>[2x]MAEVIRSSAFWRSFPIFEEFDSETLCELSGIASYRKWSAGTVIFQRGDQGDYMI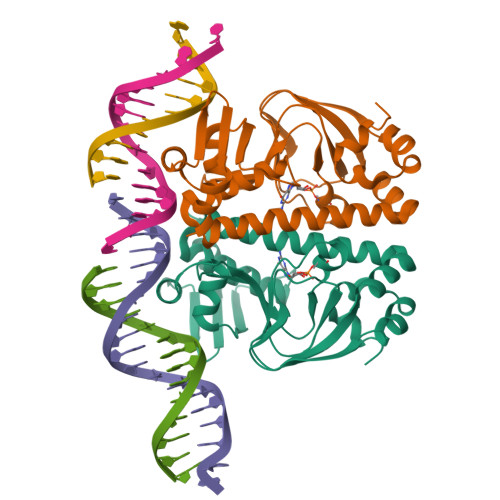VVVSGRIKLSLFTPQGRELMLRQHEAGALFGEMALLDGQPRSADATAVTAAEGYVIGKKDFLALITQRPKTAEAVIRFLCAQLRDTTDRLETIALYDLNARVARFFLATLRQIHGSEMPQSANLRLTLSQTDIASILGASRPKVNRAILSLEESGAIKRADGIICCNVGRLLSIADPEEDLEHHHHHHHH[(2R,3R,4S,5S,6R)-6-(hydroxymethyl)-2,4,5-tris(oxidanyl)oxan-3-yl]oxy-N-[9-[(2R,3S,5R)-5-[[[(2R,3S)-4-methyl-2,3-bis(oxidanyl)pentanoyl]amino]-oxidanyl-phosphoryl]oxy-3-oxidanyl-oxolan-2-yl]purin-6-yl]phosphonamidic 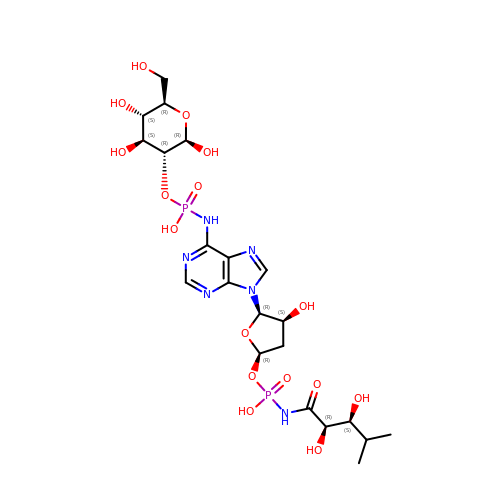acid | C21 H34 N6 O16 P2 | KOMSNTWZRZGGEF-AIJJVVIGSA-N>GSETQKKLLKDLEDKYRVSRWQPPSFKEVAGSFNLDPSELEELLHYLVREGVLVKINDEFYWHRQALGEAREVIKNLASTGPFGLAEARDALGSSRKYVLPLLEYLDQVKFTRRVG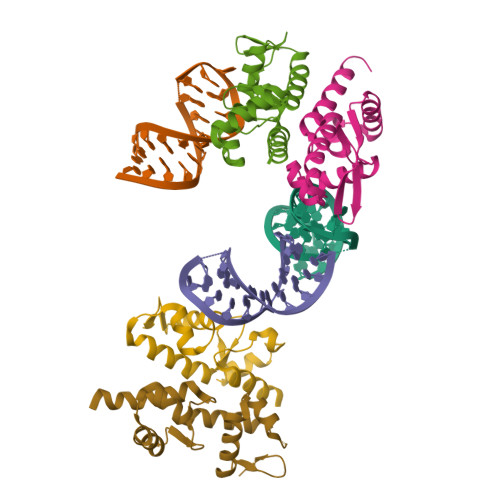DKRVVVGN[4x]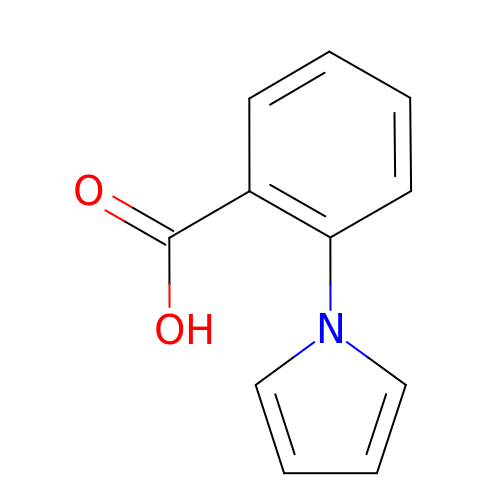2-pyrrol-1-ylbenzoic acid | C11 H9 N O2 | GNWTWXOZRSBCOZ-UHFFFAOYSA-N Among these channels, the Stelar K+ outward rectifier channel (SKOR) functions as a K+ efflux channel for long-distance distribution of K+ from roots to the upper parts of the plant. Interestingly, SKOR contains an intracellular ankyrin repeat (ANK) domain, which is absent in all the depolarization-activated K+ channels with known structure. Each protomer can be arbitrarily divided into four layers along the central axis: a transmembrane domain (TMD) comprising six transmembrane α-helices designated as S1–S6, a gating ring formed by the C-linker, a cytoplasmic domain homologous with the cyclic nucleotide-binding domain (CNBD), and an ANK domain. Unlike the canonical potassium channel, SKOR does not adopt a C4 but a C2 symmetry, which occurs in the C-linker, CNBD and ANK domain.

Besides the wild-type SKOR, we also determined the structure of an SKOR mutant L271P-D312N (SKORmut), which was reported to convert outwardly rectifying SKOR into an inward rectifier, at a resolution of 3.1 Å. Structural comparison of SKORwt1 and SKORmut showed that the pore domains of these two structures are almost identical, indicating that SKORmut is also in a closed state. Notably, our electrophysiological data demonstrated that SKORmut is a non-functional channel, rather than a converted inward rectifier, which was consistent with the closed structure in vitro.

>MGGSSGGGVSYRSGGESDVELEDYEVDDFRDGIVESRGNRFNPLTNFLGLDFAGGSGGKFTVINGIRDISRGSIVHPDNRWYKAWTMFILIWALYSSFFTPLEFGFFRGLPENLFILDIAGQIAFLVDIVLTFFVAYRDSRTYRMIYKRSSIALRYLKSTFIIDLLACMPWDIIYKAAGEKEEVRYLLLIRLYRVHRVILFFHKMEKDIRINYLFTRIVKLIFVELYCTHTAACIFYYLATTLPASQEGYTWIGSLKLGDYSYSKFREIDPWTRYTTSMYFAVVTMATVGYGDIHAVNMREMIFAMVYISFNMILGAYLIGNMTALIVKGSKTERFRDKMADIMRYMNRNKLGRNIRGQITGHLRLQYESSYTEAAVLQDIPVSIRAKIAQTLYLPYIEKVPLFRGCSSEFINQIVIRLHEEFFLPGEVIMEQGSVVDQLYFVCHGVLEEIGITKDGSEEIVAVLQPDHSFGEISILCNIPQPYTVRVAELCRILRLDKQSFMNILEIFFHDGRRILNNLLEGKESNVRIKQLESDITFHISKQEAELALKLNSAAFYGDLYQLKSLIRAGGDPNKTDYDGRSPLHLAASRGYEDITLYLIQESVDVNIKDKLGSTPLLEAIKNGNDRVAALLVKEGATLNIENAGTFLCTVVAKGDSDFLKRLLSNGIDPNSKDYDHRTPLHVAASEGFYVLAIQLVEASANVLAKDRWGNTPLDEALGCGNKMLIKLLEDAKNSQISSFPSGSKEPKDKVYKKKCTVYFSHPGDSKEKRRRGIVLWVPRSIEELIRTAKEQLNVPEASCVLSEDEAKIIDVDLISDGQKLYLAVET[4x]>GSQIHVDTMKVINDPIHGHIELHPLLVRIINTPQFQRLRYIKQLGGGYYVFPGASHNRFEHSLGVGYLAGCLVHALGEKQPELQISERDVLCVQIAGLCHDLGHGPFSHMFDGRFIPLARPEVKWTHEQGSVMMFEHLINSNGIKPVMEQYGLIPEEDICFIKEQIVGPLESPVEDSLWPYKGRPENKSFLYEIVSNKRNGIDVDKWDYFARDCHHLGIQNNFDYKRFIKFARVCEVDNELRICARDKEVGNLYDMFHTRNSLHRRAYQHKVGNIIDTMITDAFLKADDYIEITGAGGKKYRISTAIDDMEAYTKLTDNIFLEILYSTDPKLKDAREILKQIEYRNLFKYVGETQPTGQIKIKREDYESLPKEVASAKPKVLLDVKLKAEDFIVDVINMDYGMQEKNPIDHVSFYCKTAPNRAIRITKNQVSQLLPEKFAEQLIRVYCKKVDRKSLYAA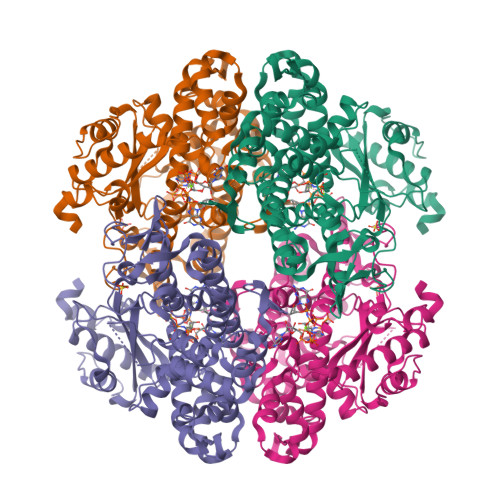RQYFVQWCADRNFTKPQDGDVIAPLITPQKKEWNDSTSVQNPTRLREASKSRVQLFKDDPM[16x]The bacterial injectisome, or type III secretion system (T3SS), is a specialized syringe-shaped protein-export system utilized by many pathogenic Gram-negative bacteria for the injection of virulence proteins (effectors) into host cells. The injectisome can be divided into three major regions: the inner- (IM) and outer-membrane (OM) spanning basal body with associated export apparatus and ATPase components, an extracellular needle, and a terminating pore inserted into the host cell membrane called the translocon. The major structural scaffold of the basal body is comprised largely of three proteins that arrange into a series of highly oligomerized, concentric rings: two intimately associated proteins localized to the IM - PrgK/EscJ/MxiJ and PrgH/EscD/MxiG, and a third protein belonging to the secretin family of OM proteins, InvG/EscC/MxiD (Salmonella enterica serovar Typhimurium SPI-1, Enteropathogenic Escherichia coli (EPEC) LEE and Shigella dysenteriae nomenclature, respectively). In summary, we report the crystal structures for the cytoplasmic and periplasmic domains of PrgH and InvG, two of the main basal body components of the prototypical Salmonella SPI-1 injectisome.

For both the cytoplasmic and periplasmic domains of PrgH, we applied a 24-mer oligomerization constraint, according to the established stoichiometry. For the cytoplasmic domain of PrgH, we observed that mutation of two leucine residues to alanine or an electronegative glutamate (Leu20 and Leu87) abrogates secretion, while a more conservative mutation to tyrosine has no effect (bottom). Negative stain EM analysis demonstrates that despite being necessary for secretion the PrgH cytoplasmic domain, as observed in a PrgH130–392 mutant (lacking the N-terminal cytoplasmic domain), is not required for assembly of the basal body. Protein sequence alignment of the PrgH orthologues indeed illustrates that the conserved residues involved in phosphopeptide binding in FHA domains are poorly conserved. To validate this, we engineered mutations of the PrgH residues corresponding to the proposed phosphothreonine interacting residues in MxiG - Arg35, Gln42 and Asp65 - to alanine. These mutations have no effect on in vivo secretion assays. We therefore conclude that the PrgH cytoplasmic domain is unlikely to interact with pThr-modified proteins. We note however that the FHA phosphopeptide interacting loops in our PrgH structure are accessible on the cytoplasmic face of the ring model, suggesting a potential interface for protein-protein interactions. Indeed, deletion of this domain results in the formation of secretion incompetent immature basal body assemblies lacking needles suggesting a role in the correct assembly/coordination of the inner-membrane export apparatus.

>PYIVRLLNSSLNGCEFPLLTGRTLFVVGQSDALTASGQLPDIPADSFFIPLDHGGVNFEIQVDTDATEIILHELKEGNSESRSVQLNTPIQVGELLILIRPESEPW[24x]>DPSKDSKAQVSAAEAGITGTWYNQLGSTFIVTAGADGALTGTYESAVGNAESRYVLTGRYDSAPATDGSGTALGWTVAWKNNYRNAHSATTWSGQYVGGAEARINTQWLLTSGTTEANAWKSTLVGHDTFTKVKPSA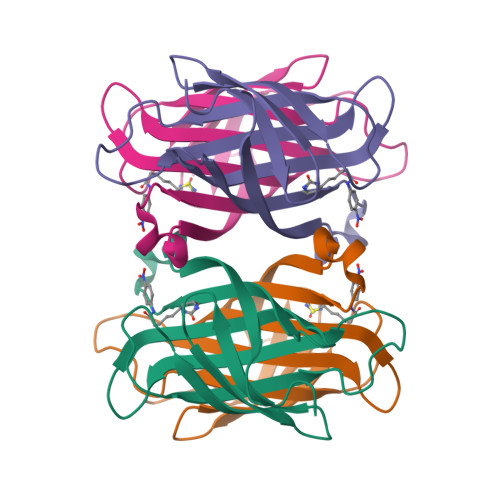AS[2x]>[6x]AEIYNKDGNKVDLYGKAVGLHYFSKGNGENSYGGNGDMTYARLGFKGETQINSDLTGYGQWEYNFQGNNSEGADAQTGNKTRLAFAGLKYADVGSFDYGRNYGVVYDALGYTDMLPEFGGDTAYSDDFFVG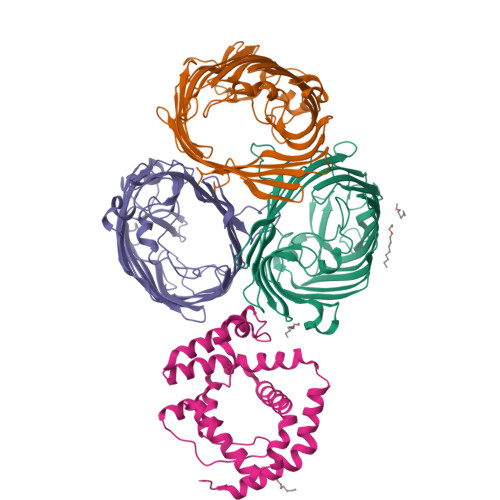RVGGVATYRNSNFFGLVDGLNFAVQYLGKNERDTARRSNGDGVGGSISYEYEGFGIVGAYGAADRTNLQEAQPLGNGKKAEQWATGLKYDANNIYLAANYGETRNATPITNKFTNTSGFANKTQDVLLVAQYQFDFGLRPSIAYTKSKAKDVEGIGDVDLVNYFEVGATYYFNKNMSTYVDYIINQIDSDNKLGVGSDDTVAVGIVYQF;>CASAPDNEPQGRSDPLEGFNRTMFDFNYNVLDPYILRPVAVAWRDYVPMPARNGISNFTSNLEEPASMVNAFLKGDPYRGMIHFNRFFLNTLLGMGGLIDVAGMANPKLAREEPNRFGSTLGHYDVGYGPYVMLPGYGSFTLRDEGGDFADTLYPMLSYLTFWMSAGKWVVEGIETRAQLLDSDGLLRNSSDPYIMVREAYFQRHDFIANGGSLKPEENPNAKAIQGELDEIDSQ[2x]>MLYEEDYKLALEAFKKVFNALTHYGAKQAFRSRARDLVEEIYNSGFIPTFFYIISKAELNSDSLDSLISLFSSDNAILRGSDENVSYSAYLFIILYYLIKRGIIEQKFLIQALRCEKTRLDLIDKLYNLAPIISAKIRTYLLAIKRLSEALIEAR[3x];>[4x]MPYYAFAEPFFIHAITHLHVGSGSSVEEEIALPFQRDELGYPTIYASSLKGAIKSFLLKEFPDKRDVIYKVLGEDENPEEASLGTFLDAILFAIPSRIIEIDSAKPYVWVYVTTYELLKKVKLYLDSISQLSNASFSNLKNKIDTILAKEGKNITLDSDLKSAILNEDFYVELEALNNKIPSIINAGVPLLVLEDSIGREVINRSLIRVRRIRIDRDKKVVETGGLWSEEYVPMKTIFFSVLLGKESKESAIFASCILRNLRYVILGGKETIGKGIVELRWVKDVI;> MKRVLIKPLEPLMFRSQGEFEPLITGSHTAAQSLIIPRPSTIAGMLGYILFNKSSGTGDWLSDLTNLLATIYGTFIETNGEYLFPLRMGNHLALVDQQHLINLPTLLEKEYERREKGIYELFYDKNKLFQIINHQDRIGISIDKSTRTVKEHYLYSARYLAFKKEVNYVIFIDNDAISDKINGKIVNFGGENRIAKLEVDDYKVDTSIEEEYYLALSPILIPDEALDNFLDNISDYVAMGKVDKISLGFDIANTKRKEMLTAILEGSIVKRSIIDFIKNEIKNDLRYRFSKYEKIGYNTLMSLCKLALRKILS;> MAIDFLVNILELIKEKQCNINLFSAISLTSIVYNNFGEFLSNNQSYSTNNPLLKYHIIILNDKNKTKDVEEKRNIFKREVAELISRNFKLDGEKVRNYFDSLKEVLKSLKYTIVDVEITTRTRALIGVSTSLGKLIFGSGISFDPYMNLPYIPASEIKGIVRSYIEGKLGEQEAEEIFGNEEREGNVNFTDAYPTRSKDFLFVPDVITPHYNGKKSEADAEPRPVIHLTIAPKVTFRFLIYYKREDVGKPICDSMPIILIRGLGARSSVGYSLFELRKIEVIKAAAHHHHHHHHHH;> MEELLMSLKLKALYPLTGGYNRHSINPFYEELVRPTEIKGLWRWWNRVLFNTLAYSTKGKLYTYESIDRLFEDVFGSENKKSAVRLEVITDEGNDNRFELSYVELDKVIDCLRNYKRKVSLDFIDNTLIAEIEGSTKIPISFKSNLDIDKIIKDLVHNNKLLSFELLGFKSVEIDATKISDKKILKEILRDLITNYLEYFNIKQEVTFTLNIYLDKSREHKQNFEDKLKFALYSLLVFILLGGIGRKTSRGFGSLSIIDVKCYDNSICKKIEDLAKNFLKISSGNELKSKIESILDCIKNSCIDTLYIENNILSEIDPKKNVVYFINSDLFEVKRINDKEKVLANIYKAVSSEGCCIKSIITDKYVRKSFLIAFGGYRKVEKDKGLDIGFIKNYLCETCETVSSFNIVDFLLSEGSFMSDYILQYEHRNSLLRFKLISDNSNNSYLIGYILHSSYFKKIDIKYVRCILEKLTYCVI;> MSIDNVLREFLDYKIIALLHDPPNKAWVITGRARNLTQQLSNIRASRKHEKVAKYIINQLFGKNYSEKVDNADKLASSIDRYLGSIVYKERSLFENRSIFLKNILLSNIQRDIGNLFPKDKSKLDNLILEYKKLLNVINKTNLILKYQLFYLIYELVWIDSKYENTPSDTRNPTHTIFDHLYATAAMMNWILSLEKEAKGYLLGIDTIGVADFISKGRKTRDLWISSYLVSALLWYVITWFIEEYGPDVILFPSLRFNQFYAFYLLEKLRKEGVSEDVIDEIKELITKYIFNGDDLFENLKIPPYPIIPGRITLILPGLIREGEEYKKVQDDNCFISKVKERYNEGWRKLIEGLRCYSERKREDGFWNLVCRVLKLTEDLLQTTPLNIRVKQVSVTEDEIFNNNKLRSDSWKIYDNKYRQLVSEFKKSKLVKVTPESRLKLFELTKFDKLPQIGEKSKRGYEFCTSCGVLPAVVIMPKEDELEKKLIDLGIARDEKDVRSIKNMISPGERLCPWCLVKRALGAEPRLMRIL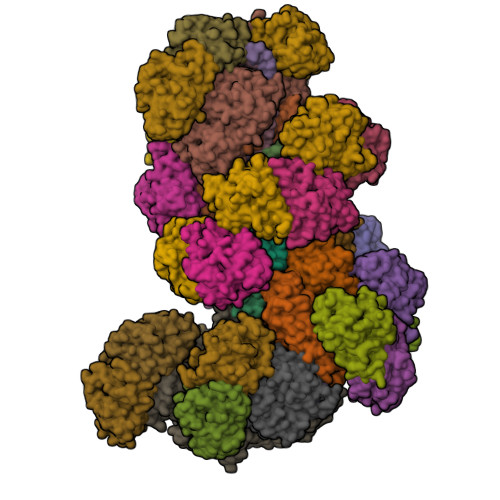LLGDLYSVEKIVNEIVSRDVKIEIPSTSDIASIKTFEEMIEKKNEICEDLKEEEVCEKPSESVLSMWQWFNKNYYNGINLTIDPEEYWFSEKRRRYYFSVFRRHRITFPSPYYALVRADSDYLGDLLEGKLTPYLAGIIDSGDYANISEKKEEVNKLLEEYLVNAGSGSIVDYVKTVLKCIRENLNKCSCAEKIYSNEVAKVMFRVNVEKANVEEEVKNSLEYFETILNEGRIIVTPAWHVSISSALNRGLLVELELVNKHKGFVIYAGGDDLLAMLPVDEVLDFIKESRRAFAGFGTEKLGNMCLENGFVRINNAYYPSLPIVGRSYSVIIAHYADPLFFVINDSYNLLEEGKEIIRYRVMYNGEYKDAKKDVAIFRYQGLTSVIPLSLKRPIVSSVSDFNEIASIIDVILELKKRIDEGRISVSLLYDYEKYKHLIVASDEKYLTEFLVKDWIKRNSLRKHVEFTIDEKLYGVRLTIENYPIKIPNDLISNIVYTLRIIYGGEK;>MSTQREYVFIPITNSITIDVKITIGGSDHITNIDERGIHNVLVITGYAVDEKNGRLVPTLDPCDYVKGILVAGTPQQAQSNDFLTLKLPANKLYLIRKKGNISDDLKIYIPYSSPDARNSMKTKPVSISDDTIVNNIIKEVFDKIYNITQKEKVKIEKVKEDIKELFSYYALEQ[26x]>[8x]MKKWLYIFILFLVAGLGSTSSADAKMPGEKSVNVSKLNVDEFFKDRDGTFILHDVQKDKTFIYNESRAKERQTPQSTFKVPNALIGLQVKAVRDEYDVKRWDGTEREFESWNRDHTLGSAMRDSVIWYYQAMARDIGEDRMKDWLHRISYGNEDISGGIDQFWLQSSLKISPLEEKDFIEHLYKEDLPFDKPIMKTVKRMMIQEEGDHYTLY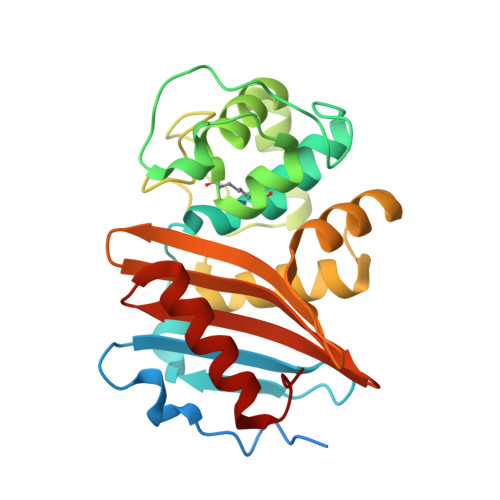GKTGTDYGLGWFVGFITTDNHSYIFVTNVDASGTAAKNITTDILKKYHLITN> SNADAESLFREALSNKVDELAHFLLRKYRAKELVTKAEMLERVIKNYKRCFPVIFGKASESLK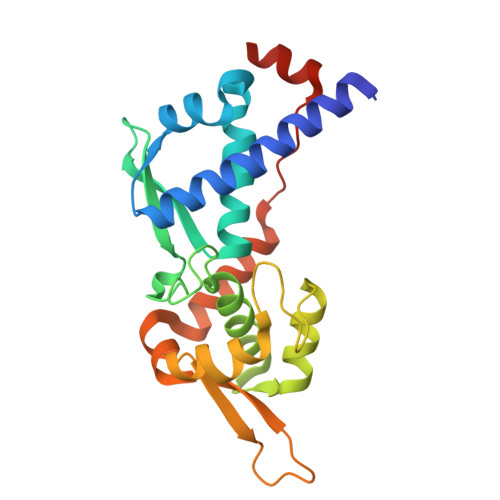MIFGIDVKEVDPTSNTYTLVTCLGLSYDGLLGNNQIFPKTGLLIIVLGTIAMEGDSASEEEIWEELGVMGVYDGREHTVYGEPRKLLTQDWVQENYLEYRQVPGSNPARYEFLWGPRALAETSYVKVLEHVVRVNARVRIAYPSLREAALLEEEEGV>[2x]SNAMLRRLFKKKYVCVRQYDLTDC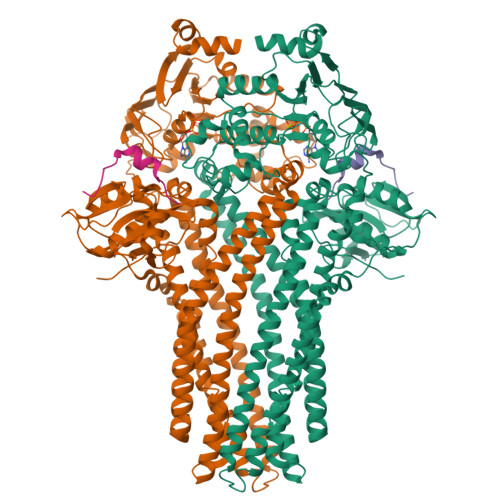GAACLSSIAQYYGLKMSLAKIREMTGTDTQGTNAYGLIHAAKQLGFSAKGVKASKEDLLKDFRLPAIANVIVDNRLAHFVVIYSIKNRIITVADPGKGIVRYSMDDFCSIWTGGLVLLEPGEAFQKGDYTQNMMVKFAGFLKPLKKTVLCIFLASLLYTALGIAGSFYIKFLFDDLIKFEKLNDLHIISAGFAVIFLLQIFLNYYRSILVTKLGMSIDKSIMMEYYSHVLKLPMNFFNSRKVGEIISRFMDASKIRQAISGATLTIMIDTIMAVIGGILLYIQNSSLFFISFIIILLYGIIVTVFNKPIQNANRQIMEDNAKLTSALVESVKGIETIKSFGAEEQTEKSTRDKIETVMKSSFKEGMLYINLSSLTGIVAGLGGIVILWAGAYNVIKGNMSGGQLLAFNALLAYFLTPVKNLIDLQPLIQTAVVASNRLGEILELATEKELREDSDDFVISLKGDIEFRNVDFRYGLRKPVLKNINLTIPKGKTVAIVGESGSGKTTLAKLLMNFYSPEKGDILINGHSIKNISLELIRKKIAFVSQDVFIFSGTVKENLCLGNENVDMDEIIKAAKMANAHDFIEKLPLKYDTFLNESGANLSEGQKQRLAIARALLKKPDILILDEATSNLDSITENHIKDAIYGLEDDVTVIIIAHRLSTIVNCDKIYLLKDGEIVESGSHTELIALKGCYFKMWKQTENTLAS;>[2x]SNAMSEAKKLNIGRELTDEELMEMTGGSTFSIQCQKDYTYKPSLPVVKYGVVIDEPEVVIKYGVGPIVGIKYGVEPIGPIQPMYGIKPVETLK> GAMAAEMDWDKTVGAAEDVRRI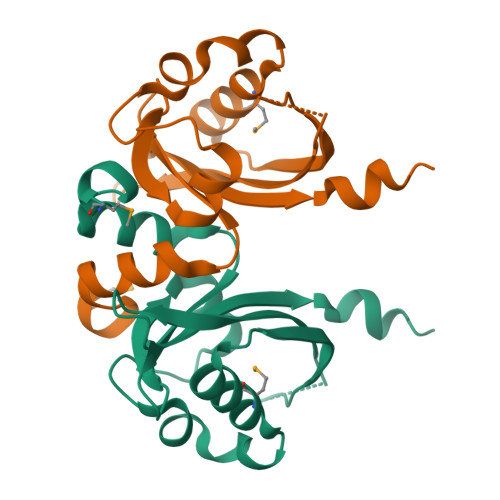FEHIPAILVGLEGPDHRFVAVNAAYRGFSPLLDTVGQPAREVYPELEGQQIYEMLDRVYQTGEPQSGSEWRLQTDYDGSGVEERYFDFVVTPRRRADGSIEGVQLIVDDVTSRVRARQAAEARVEEL>MHHHHHHENLYFQTNPEALTVAATEVRRIRDRAIQSDAQVAPMTTAVRPPAADLVSEKAATFL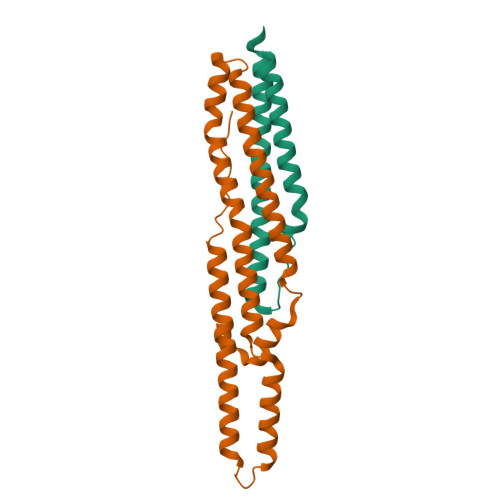VEYARKYRQTIAAAAVVLEEFAHALTTGADKYATAEADNIKTFS[2x];>[2x]MHFEAYPPEVNSANIYAGPGPDSMLAAARAWRSLDVEMTAVQRSFNRTLLSLMDAWAGPVVMQLMEAAKPFVRWLTDLCVQLSEVERQIHEIVRAYEWAHHDMVPLAQIYNNRAERQILIDNNALGQFTAQIADLDQEYDDFWDEDGEVMRDYRLRVSDALSKLTPWKAPPPIA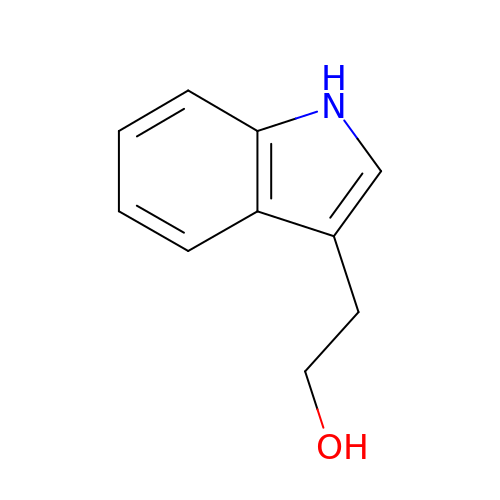2-(1H-indol-3-yl)ethanol | C10 H11 N O | MBBOMCVGYCRMEA-UHFFFAOYSA-N>[4x]MSQHNEKNPHQHQSPLHDSSEAKPGMDSLAPEDGSHRPAAEPTPPGAQPTAPGSLKAPDTRNEKLNSLEDVRKGSENYALTTNQGVRIADDQNSLRAGSRGPTLLEDFILREKITHFDHERIPERIVHARGSAAHGYFQPYKSLSDITKADFLSDPNKITPVFVRFSTVQGGAGSADTVRDIRGFATKFYTEEGIFDLVGNNTPIFFIQDAHKFPDFVHAVKPEPHWAIPQGQDAHDTFWDYVSLQPETLHNVMWAMSDRGIPRSYRTMEGFGIHTFRLINAEGKATFVRFHWKPLAGKASLVWDEAQKLTGRDPDFHRRELWEAIEAGDFPEYELGFQLIPEEDEFKFDFDLLDPTKLIPEELVPVQRVGKMVLNRNPDNFFAENEQAAFHPGHIVPGLDFTNDPLLQGRLFSYTDTQISRLGGPNFHEIPINRPTCPYHNFQRDGMHRMGIDTNPANYEPNSINDNWPRETPPGPKR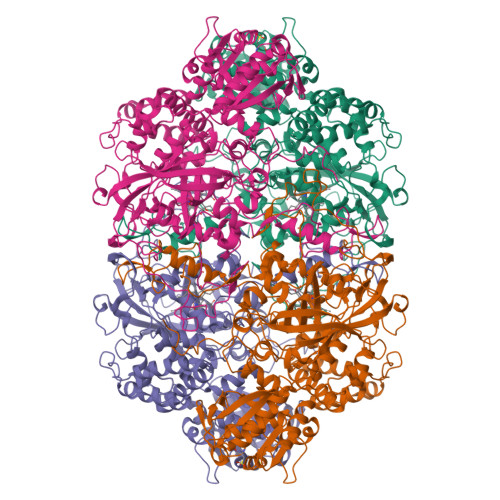GGFESYQERVEGNKVRERSPSFGEYYSHPRLFWLSQTPFEQRHIVDGFSFELSKVVRPYIRERVVDQLAHIDLTLAQAVAKNLGIELTDDQLNITPPPDVNGLKKDPSLSLYAIPDGDVKGRVVAILLNDEVRSADLLAILKALKAKGVHAKLLYSRMGEVTADDGTVLPIAATFAGAPSLTVDAVIVPCGNIADIADNGDANYYLMEAYKHLKPIALAGDARKFKATIKIADQGEEGIVEADSADGSFMDELLTLMAAHRVWSRIPKIDKIPA(2~{R},3~{R},4~{S},5~{R})-2-(6-aminopurin-9-yl)-5-[[3-[6-azanyl-9-[(2~{R},3~{R},4~{S},5~{R})-5-(hydroxymethyl)-3,4-bis(oxidanyl)oxolan-2-yl]purin-8-yl]prop-2-ynylamino]methyl]oxolane-3,4-diol 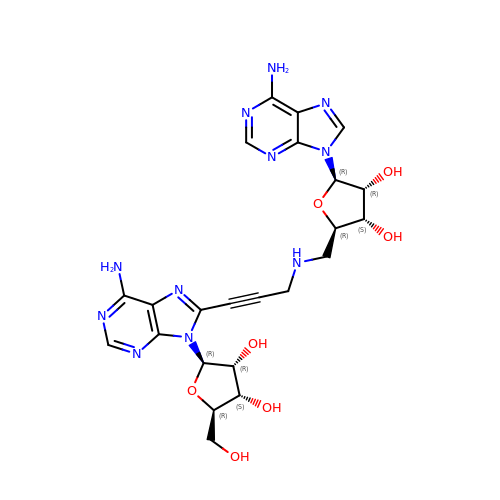| C23 H27 N11 O7 | CGSYXPCXDPYUKS-MKWZPUSRSA-N>[3x]MSDEKIINQPQDVVSEMLDGLTYAYGDLIEKVPDFEIIQRKSPKSGKVALVSGGGSGHEPAHAGFVGEGMLSAAVCGAIFTSPTPDQIYEAIKSADEGAGVLLIIKNYLGDVMNFEMAREMAEMEEIKVEQIIVDDDIAVENSLYTQGRRGVAGTVLVHKILGAAAHQEASLDEIKDLADKVVKNIKTIGLALSAATVPEVGKPGFVLDDN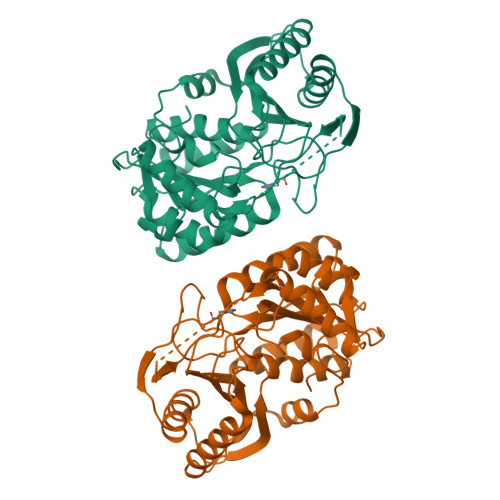EIEYGVGIHSEPGYRREKMKTSYELATELVGKLKEEFKFEAGQKYGILVNGMGATPLMEQFIFMNDVAKLLTEENIEILFKKVGNYMTSIDMAGLSLTMIKLEDDQWLKNLNEDVKTISWG>[3x]AQV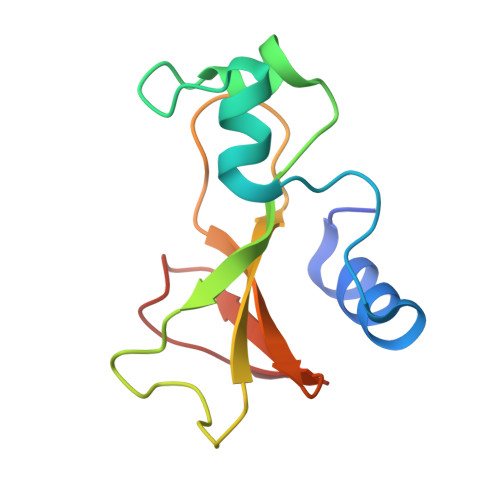INTFDGVADYLQTYHKLPDNYITKSEAQALGWVASKGNLADVAPGKSIGGDIFSNREGKLPGKSGRTWREADINYTSGFRNSDRILYSSDWLVYKTTDHYQTFTKIR>GSHMSETASWQPSASIPNLLKRAAIMAEIRRFFADRGVLEVETPCMSQATVTDIHLVPFETRFVGPGHSQGMNLWLMTSPEYHMKRLLVAGCGPVFQLCRSFRNEEMGRYHNPEFTMLEWYRPHYDMYRLMNEVDDLLQQVLDCPAAESLSYQQAFLRYLEIDPLSADKTQLREVAAKLDLSNVADTEEDRDTLLQLLFTFGVEPNIGKEKPTFVYHFPASQASLAQISTEDHRVAERFEVYYKGIELANGFHELTDAREQQQRFEQDNRKRAARGLPQHPIDQNLIEALKVGMPDCSGVALGVDRLVMLALGAETLAEVIAFSVDRA[4x];>GSHMATYYSNDFRAGLKIMLDGEPYAVEASEFVKPGKGQAFARVKLRRLLTGTRVEKTFKSTDSAEGADVVDMNLTYLYNDGEFWHFMNNETFEQLSADAKAIGDNAKWLLDQAECIVTLWNGQPISVTPPNFVELEIVDTDPGLKGDTAGTGGKPATLSTGAVVKVPLFVQIGEVIKVDTRSGEYVSRV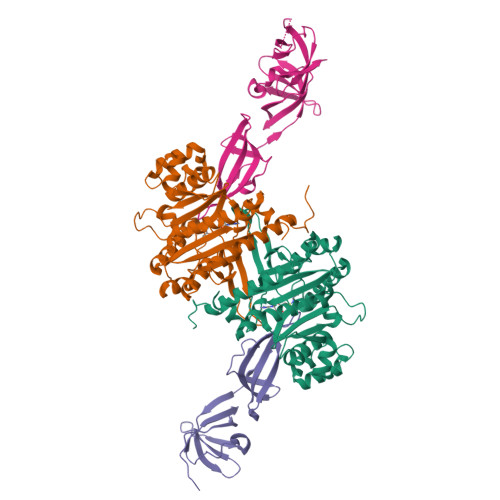K[4x]> GTGPDKLKKVLDKLRLKRKDISEAAETVNKVVERLLRRMQKRESEFKGVEQLNTGSYYEHVKISAPNEFDVMFKLEVPRIELQEYYETGAFYLVKFKRIPRGNPLSHFLEGEVLSATKMLSKFRKIIKEEVKEIKDIDVSVEKEKPGSPAVTLLIRNPEEISVDIILALESKGSWPISTKEGLPIQGWLGTKVRTNLRREPFYLVPKNAKDGNSFQGETWRLSFSHTEKYILNNHGIEKTCCESSGAKCCRKECLKLMKYLLEQLKKEFQELDAFCSYHVKTAIFHMWTQDPQDSQWDPRNLSSCFDKLLAFFLECLRTEKLDHYFIPKFNLFSQELIDRKSKEFLSKKIEYERNNGFPIFDKL

Cyclic GMP-AMP (cGAMP) synthase (cGAS) is essential for the host defense against cytosolic double-stranded (ds)DNA arising from various maladies (e.g., pathogen invasion, ionizing irradiation, and genotoxic chemicals). Upon directly binding to and dimerizing on dsDNA, cGAS cyclizes ATP and GTP into 2′−5′/3′−5′-linked cGAMP, a unique metazoan second messenger for initiating type-I interferon (IFN-I)-mediated inflammatory responses. cGAS is central to antitumor immunity, host defense against an array of pathogens, and regulating autoimmunity. Here, we resolve these numerous fundamental mechanistic questions in innate immunology and present a unifying catalytic mechanism of cGAS. Finally, we reveal how mouse cGAS achieves more stringent substrate selectivity and higher catalytic efficiency than the human enzyme. Together, we set forth a unifying catalytic mechanism of cGAS in which dsDNA-binding pre-organizes the active site into a rigid yet adaptable lock for two sets of keys (substrates and intermediate) necessary to specifically synthesize 2′−5/3′−5′-cGAMP.

We next solved the crystal structure of ATP-bound mcGAScat without dsDNA via soaking. Here, one ATP was clearly bound at its designated binding pocket (Site-1), but the second NTP binding site (Site-2) remained empty (i.e., the GTP binding site). Strikingly, electron densities were missing for both the ribose of ATP and Mg2+; the catalytic residues stayed in the inactive state and the triphosphate appeared suboptimal for coordinating Mg2+. G dsDNA-free WT-mcGAScat bound to ATP. The ribose was modeled without density for presentation. Considering that the ribose of bound ATP was unresolved without dsDNA, we hypothesized that these interactions underpin productive substrate binding, which would also allow cGAS to discriminate against deoxy(d)-ATP.>GSAAAQDMVSPPPP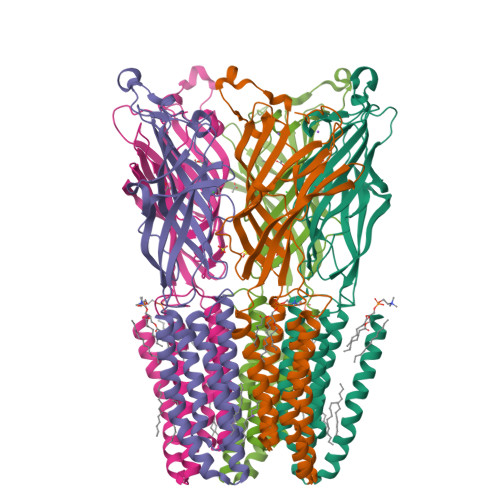IADEPLTVNTGIYLIECYSLDDKAETFKVNAFLSLSWKDRRLAFDPVRSGVRVKTYEPEAIWIPEIRFVNVENARDADVVDISVSPDGTVQYLERFSARVLSPLDFRRYPFDSQTLHIYLIVRSVDTRNIVLAVDLEKVGKNDDVFLTGWDIESFTAVVKPANFALEDRLESKLDYQLRISRQYFSYIPNIILPMLFILFISWTAFWSTSYEANVTLVVSTLIAHIAFNILVETNLPKTPYMTYTGAIIFMIYLFYFVAVIEVTVQHYLKVESQPARAASITRASRIAFPVVFLLANIILAFLFFG[5x]> ATITQDTPINQIFTDTALAEKMKTVLGKTNVTDTVSQTDLDQVTTLQADRLGIKSIDGVEYLNNLTQINFSNNQLTDITPLKNLTKLVDILMNNNQIADITPLANLTNLTGLTLFNNQITDIDPLKNLTNLNRLELSSNTISDISALSGLTSLQQLSFSSNQVTDLKPLANLTTLERLDISSNKVSDISVLAKLTNLESLIATNNQISDITPLGILTNLDELSLNGNQLKDIGTLASLTNLTDLDLANNQISNLAPLSGLTKLTELKLGANQISNISPLAGLTALTNLELNENQLEDISPISNLKNLTYLTLYFNNISDISPVSSLTKLQRLFFYNNKVSDVSSLANLTNINWLSAGHNQISDLTPLANLTRITQLGLNDQAW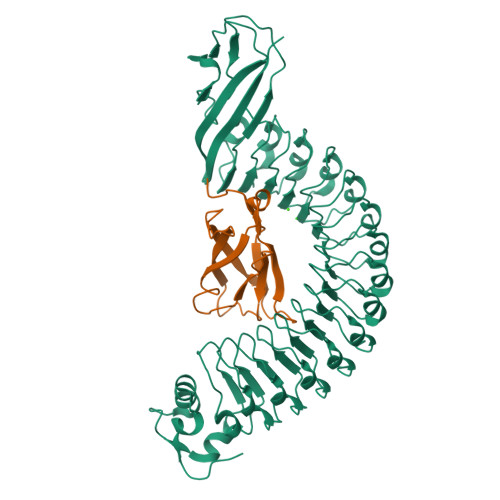TNAPVNYKANVSIPNTVKNVTGALIAPATISDGGSYTEPDITWNLPSYTNEVSYTFSQPVTIGKGTTTFSGTVTQPLKA;> GPLGSWVIPPISCPENEKGPFPKNLVQIKSNKDKEGKVFYSITGQGADTPPVGVFIIERETGWLKVTEPLDRERIATYTLFSHAVSSNGNAVEDPMEILITVTDQ2-methylpropanal 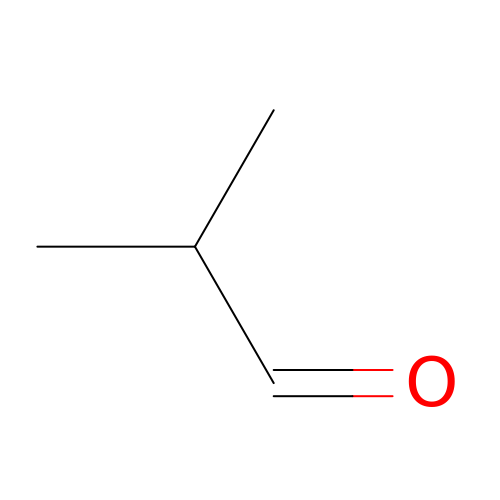| C4 H8 O | AMIMRNSIRUDHCM-UHFFFAOYSA-N>[5x]MAWPKVQPEVNIGVVGHVDHGKTTLVQAITGIWTSKHSEELKRGMTIKLGYAETNIGVCESCKKPEAYVTEPSCKSCGSDDEPKFLRRISFIDAPGHEVLMATMLSGAALMDGAILVVAANEPFPQPQTREHFVALGIIGVKNLIIVQNKVDVVSKEEALSQYRQIKQFTKGTWAENVPIIPVSALHKINIDSLIEGIEEYIKTPYRDLSQKPVMLVIRSADVNAPGTQ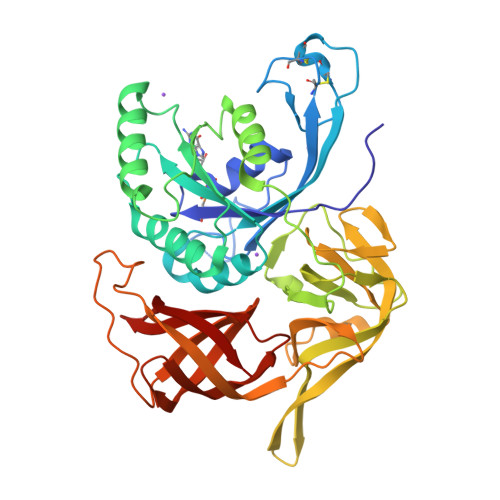FNELKGGVIGGSIIQGLFKVDQEIKVLPGLRVEKQGKVSYEPIFTKISSIAFGDEEFKEAKPGGLVAIGTYLDPSLTKADNLLGSIITLADAEVPVLWNIRIKYNLLERVVGAKEMLKVDPIRAKETLMLSVGSSTTLGIVTSVKKDEIEVELRRPVAVWSNNIRTVISRQIAGRWRMIGWGLVEI> MAFEALTGINGDLITRSWSASKQAYLTERYHKEEAGAVVIFAFQPSFSEKDFFDPDNKSSFGEIKLNRVQFPCMRKIGKGDVATVNEAFLKNLEAIIDPRTSFQASVEMAVRSRKQIVFTGHSSGGATAILATVWYLEKYFIRNPNVYLEPRCVTFGAPLVGDSIFSHALGREKWSRFFVNFVSRFDIVPRIMLARKASVEETLPHVLAQLDPRKSSVQESEQRITEFYTRVMRDTSTVANQAVCELTGSAEAFLETLSSFLELSPYRPAGTFVFSTEKRLVAVNNSDAILQMLFYTSQASDEQEWSLIPFRSIRDHHSYEELVQSMGKKLFNHLDGENSIESTLNDLGVSTRGRQYVQAALEEEKKRVENQKKIIQVIEQERFLKKLAWIEDEYKPKCQAHKNGYYDSFKVSNEENDFKANVKRAELAGVFDEVLGLMKKCQLPDEFEGDIDWIKLATRYRRLVEPLDIANYHRHLKNEDTGPYMKRGRPTRYIYAQRGYEHYILKPNGMIAEDVFWNKVNGLNLGLQLEEIQ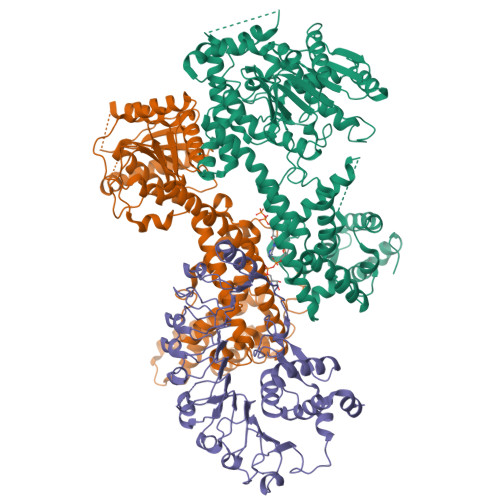ETLKNSGSECGSCFWAEVEELKGKPYEEVEVRVKTLEGMLGEWITDGEVDDKEIFLEGSTFRKWWITLPKNHKSHSPLRDYMMDEITDT;> MESSSSLKGSALGKLVVTSGLLHSSWSKILEIHNPPYSNHDPGLQVSKKKKDSGLEFQIHREEKFTLVVFSAPPICRSSSSDSTLLHVKDKENPFPFLCSENNPSFSLHTPAFNLFTSASTSLTYLKSELLQTLKSEKPVIITGAALGGSVASLYTLWLLETIEPTLKRPLCITFGSPLIGDASLQQILENSVRNSCFLHVVSAQTRIKMDFFKPFGTFLICFDSGCVCIEDHVAVTELLNGVHDSGLVDYSQVLNRLDQSMLSLADSRLIPEDVIKGIEKRAEMKNLRFDMMFKKLNDMKISMAYIEWYKKKCKEVKIGYYDRFKTQLAFPSKEFDINIKNHHKSELNRFWKSVVEEVERRPQSDASILKRRFLFSGNNYRRMIEPLDIAEYYLEGRKEYRTTGRSHHYVMLEKWFGMESILIEKERCKKRDLSDLLTFDSCFWAEVEDSLIVINQLNTTVGMRDDVREVLTRKLVEFEGYVWEIITKREVSPEIFLEESSFMKWWKEYKKIKGFNSSYLTEFMNTRKYESYGKSQ;> MNDWASLGIGSIGEAVFSKLLKVVIDEAKKFKAFKPLSKDLVSTMEILFPLTQKIDSMQKELDFGVKELKELRDTIERADVAVRKFPRVKWYEKSKYTRKIERINKDMLKFCQIDLQLLQHRNQLTLLGLTGNEVNSVDGLSKRMDLLSVPAPVFRDLCSVPKLDKVIVGLDWPLGELKKRLLDDSVVTLVVSAPPGCGKTTLVSRLCDDPDIKGKFKHIFFNVVSNTPNFRVIVQNLLQHNGYNALTFENDSQAEVGLRKLLEELKENGPILLVLDDVWRGADSFLQKFQIKLPNYKILVTSRFDFPSFDSNYRLKPLEDDDARALLIHWASRPCNTSPDEYEDLLQKILKRCNGFPIVIEVVGVSLKGRSLNTWKGQVESWSEGEKILGKPYPTVLECLQPSFDALDPNLKECFLDMGSFLEDQKIRASVIIDMWVELYGKGSSILYMYLEDLASQNLLKLVPLGTNEHEDGFYNDFLVTQHDILRELAICQSEFKENLERKRLNLEILENTFPDWCLNTINASLLSISTDDLFSSKWLEMDCPNVEALVLNLSSSDYALPSFISGMKKLKVLTITNHGFYPARLSNFSCLSSLPNLKRIRLEKVSITLLDIPQLQLSSLKKLSLVMCSFGEVFYDTEDIVVSNALSKLQEIDIDYCYDLDELPYWISEIVSLKTLSITNCNKLSQLPEAIGNLSRLEVLRLCSSMNLSELPEATEGLSNLRFLDISHCLGLRKLPQEIGKLQNLKKISMRKCSGCELPESVTNLENLEVKCDEETGLLWERLKPKMRNLRVQEEEIEHNLNLLQMF>[2x]MDLADRFAELERRYDARLGVYVPATGTTAAIEYRADERFAFCSTFKAPLVAAVLHQNPLTHLDKLITYTSDDIRSISPVAQQHVQTGMTIGQLCDAAIRYSDGTAANLLLADLGGPGGGTAAFTGYLRSLGDTVSRLDAEEP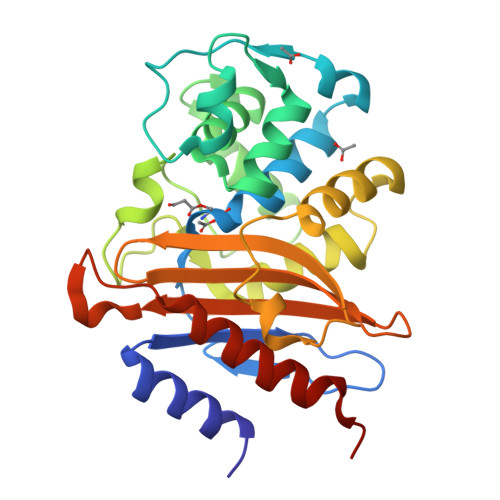ELNRDPPGDERDTTTPHAIALVLQQLVLGNALPPDKRALLTDWMARNTTGAKRIRAGFPADWKVIDKTGTGDYGRANDIAVVWSPTGVPYVVAVMSDRAGGGYDAEPREALLAEAATCVAGVLALEHHHHHH> EGVSNLVGLPNNICLQKTSNQILKPKLISYTLPVVGQSGTCITDPLLAMDEGYFAYSHLERIGSCSRGVSKQRIIGVGEVLDRGDEVPSLFMTNVWTPPNPNTVYHCSAVYNNEFYYVLCAVSTVGDPILNSTYWSGSLMMTRLAVKPKSNGGGYNQHQLALRSIEKGRYDKVMPYG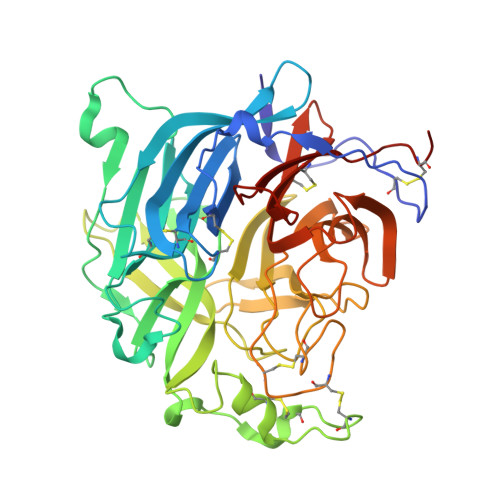PSGIKQGDTLYFPAVGFLVRTEFKYNDSNCPITKCQYSKPENCRLSMGIRPNSHYILRSGLLKYNLSDGENPKVVFIEISDQRLSIGSPSKIYDSLGQPVFYQASFSWDTMIKFGDVLTVNPLVVNWRNNTVISRPGQSQCPRFNTCPEICWEGVYNDAFLIDRINWISAGVFLDSNQTAENPVFTVFKDNEILYRAQLASEDTNAQKTITNCFLLKNKIWCISLVEIYDTGDNVIRPKLFAVKIPEQCTA>AMEQLLRAELRTATLRAFGGPGAGCISEGRAYDTDAGPVFVKVNRRTQARQMFEGEVASLEALRSTGLVRVPRPMKVIDLPGGGAAFVMEHLKMKSLSSQASKLGEQMADLHLYNQKGSSYVDKFGFHTVTCCGFIPQVNEWQDDWPTFFARHRLQAQLDLIEKDYADREARELWSRLQVKIPDLFCGLEIVPALLHGDLWSGNVAEDDVGPIIYDPASFYGHSEFELAIALMFGGFPRSFFTAYHRKIPKAPGFDQRLLLYQLFNYLNHWNHFGREYRSPSLGTMRRLLK[2x]

Glycation, a non-enzymatic post-translational modification occurring on proteins, can be actively reversed via site-specific phosphorylation of the fructose-lysine moiety by FN3K kinase, to impact the cellular function of the target protein. Alternatively, the sugar moiety on glycated residues can be phosphorylated by a class of small-molecule kinases called fructosamine-3-kinases (FN3Ks), which are present in mammals, birds, and plants. Further characterization indicated that FN3K is responsible for protein deglycation by phosphorylating protein-associated fructosamines. Here, we determined a series of crystal structures of HsFN3K in the apo-state, and in complex with different nucleotide analogs together with a sugar substrate mimic to reveal the features important for its kinase activity and substrate recognition.

To investigate the structural basis of FN3K kinase activity, we determined a crystal structure of HsFN3K in its apo state. We, therefore, designed an internal loop truncated HsFN3K (HsFN3K∆) guided by limited proteolysis experiments. HsFN3K∆ crystallized in space group P212121 with two molecules in the asymmetric unit (ASU). The whole HsFN3K∆ polypeptide could be unambiguously traced in the 1.67 Å resolution electron density map, revealing a globular bi-lobal structure with the N-lobe and C-lobe exhibiting a canonical protein-kinase-like (PKL)-fold. The two C-lobes in the ASU are placed in a head-to-head orientation with the N-lobe α1 helix from one protomer positioned onto the N-lobe β-sheet of the second, forming a domain-swapped dimer. The dimeric arrangement of the two HsFN3K protomers is supported by an intermolecular di-sulfide linkage between the side chain of a Cys24 residue from the ATP-binding P-loop of each protomer. The electrostatic surface of the Apo-HsFN3K structure exhibits an overall negatively charged pocket, decorated with polar residues, near the P-loop for ATP binding, and a sulfate ion is observed in one protomer occupying the space for the nucleotide β-phosphate in this structure. Adjacent to it, the substrate binding pocket is also negatively charged and is decorated with polar residues. Notably, in contrast to a fully extended conformation of the P-loop in AtFN3K, the P-loop in HsFN3K packs against the N-lobe β-sheet. Apo-HsFN3K has an overall PKL kinase fold, and although it was purified under reducing conditions as a primarily monomeric protein in solution, it forms a domain-swapped dimer supported by an intermolecular disulfide bond in the P-loop in the crystal structure.> GSPCVEVVPNITYQCEELNFYKIPDNLPFSTKNLDLSFNPLRHLGSYSFFSFPELQVLDLSRCEIQTIEDGAYQSLSHLSTLILTGNPIQSLALGAFSGLSSLQKLVAVETN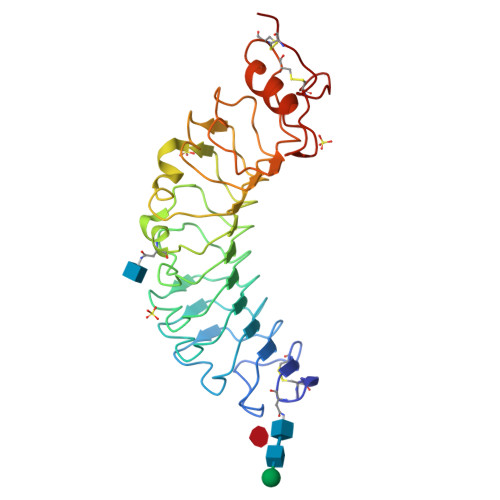LASLENFPIGHLKTLKELNVAHNLIQSFKLPEYFSNLTNLEHLDLSSNKIQSIYCTDLRVLHQMPLLNLSLDLSLNPMNFIQPGAFKEIRLKELALDTNQLKSVPDGIFDRLTSLQKIWLHTNPWDCSCPRIDYLSRWLNKNSQKEQGSAKCSGSGKPVRSIICPT>QPRPAFSAIRRNPPMGGNVVIFDTVITNQEEPYQNHSGRFVCTVPGYYYFTFQVLSQWEI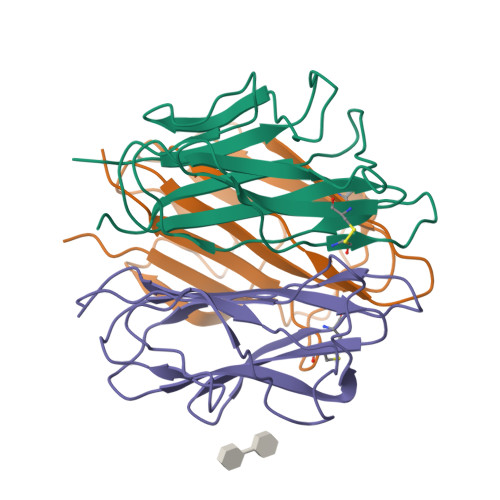CLSIVSSSRGQVRRSLGFCDTTNKGLFQVVSGGMVLQLQQGDQVWVEKDPKKGHIYQGSEADSVFSGFLIFPSA[2x];>ATQKIAFSATRTINVPLRRDQTIRFDHVITNMNNNYEPRSGKFTCKVPGLYYFTYHASSRGNLCVNLMRGRERAQKVVTFCDYAYNTFQVTTGGMVLKLEQGENVFLQATDKNSLLGMEGANSIFSGFLLFPDMEA[2x];>KQKFQSVFTVTRQTHQPPAPNSLIRFNAVLTNPQGDYDTSTGKFTCKVPGLYYFVYHASHTANLCVLLYRSGVKVVTFCGHTSKTNQVNSGGVLLRLQVGEEVWLAVNDYYDMVGIQGSDSVFSGFLLFPD[2x]> MAMYQQYSPKDVVCSWNGIAIEGFAPDSFLRLQRTSPLVTPVVGAGGQVALTRNADKTGTIEIELMQTSLS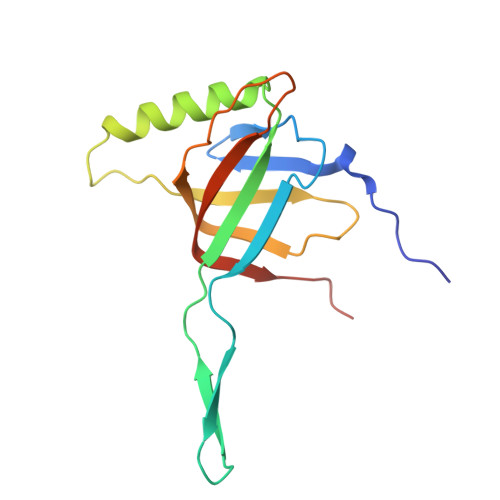NQMLSAIQAKQDNMELEEDISSNFVIYDPSGSVLATGINAWLQELPQIELGRDQNSKTWIFGCEKLDYTSTIPASSV(2S)-N-(4-Methoxybenzyl)tetrahydrofuran-2-carboxamide | C13 H17 N O3 | 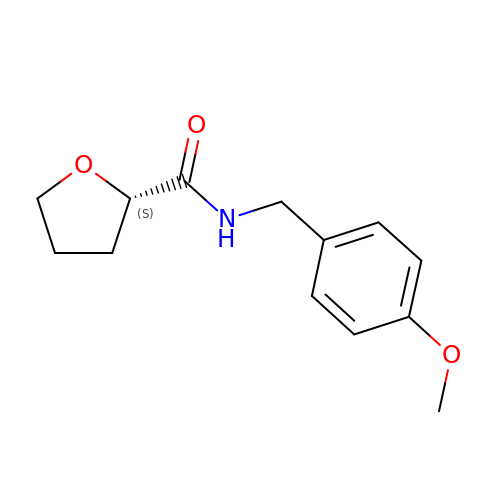VUHXHMGNBINEHD-LBPRGKRZSA-N>[3x]GAMNNTIINSLIGGDDSIKRSNVFAVDSQIPTLYMPQYISLSGVMTNDGPDNQAIASFEIRDQYITALNHLVLSLELPEVKGMGRFGYVPYVGYKCINHVSISSCNGVIWEIEGEELYNNCINNTIALKHSGYSSELNDISIGLTPNDTIKEPSTVYVYIKTPFDVEDTFSSLKLSDSKITVTVTFNPVSDIVIRDSSFDFETFNKEFVYVPELSFIGYMVKNVQIKPSFIEKPRRVIGQINQPTAT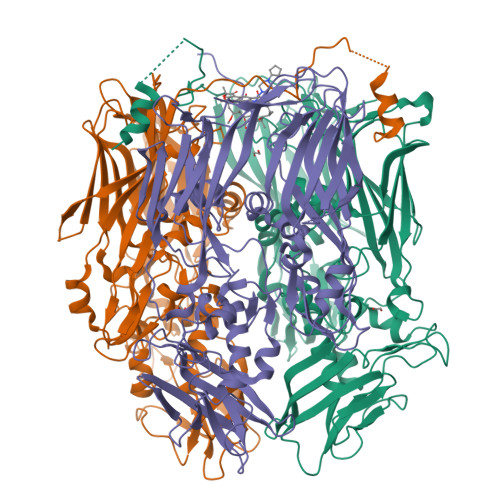VTEVHAATSLSVYTKPYYGNTDNKFISYPGYSQDEKDYIDAYVSRLLDDLVIVSDGPPTGYPESAEIVEVPEDGIVSIQDADVYVKIDNVPDNMSVYLHTNLLMFGTRKNSFIYNISKKFSAITGTYSDATKRTIFAHISHSINIIDTSIPVSLWTSQRNVYNGDNRSAESKAKDLFINDPFIKGIDFKNKTDIISRLEVRFGNDVLYSENGPISRIYNELLTKSNNGTRTLTFNFTPKIFFRPTTITANVSRGKDKLSVRVVYSTMDVNHPIYYVQKQLVVVCNDLYKVSYDQGVSITKIMGDNN2-AMINO-P-CRESOL 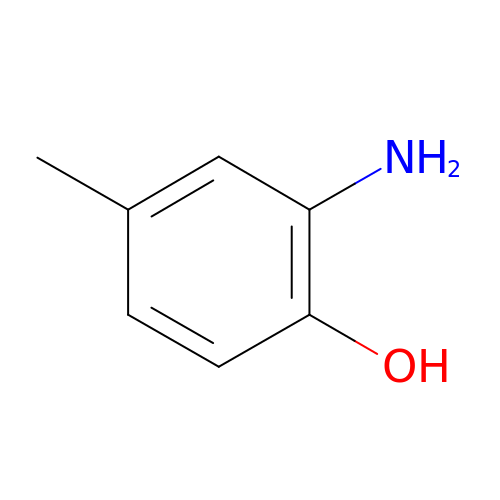| C7 H9 N O | ZMXYNJXDULEQCK-UHFFFAOYSA-N A-1(L) is a Myoviridae cyanophage isolated in 1970s9 that specifically infects the model cyanobacterium Anabaena sp. PCC 7120. Using cryo-electron microscopy (cryo-EM), we solved the structure of A-1(L) tail machine, which consists of three parts: a 205-Å-long neck, a 1045-Å-long contractile tail with a complicated baseplate, and six pairs of tail fibers. The dodecameric gp2 portal, the pentadecameric gp5 and the hexameric gp7 sequentially constitute the neck of A-1(L), to which five neck fibers are attached. The long and contractile tail of A-1(L) contains 24 rings of gp10 hexamers that form the tube, surrounded by the sheath of 24 helically stacked gp9 hexamers.

The central spike/trimeric gp25, hub/trimeric gp15, six monomeric gp16, and six wedges/heterotrimeric (gp31)2-gp32 form a compact baseplate at the distal end of the tail. The central spike locates at the innermost of baseplate, each subunit of which adopts a conserved structure: an N-terminal α-helix, an oligonucleotide/oligosaccharide binding fold, a consecutive β-strand domain and a C-terminal loop. The N-terminal α-helices (residues Met1-Arg30) of three gp25 subunits form a tripod to interwind with the tripod of three C-terminal helices (residues Pro666-Ala689) of TMP via hydrogen bonds and hydrophobic interactions. The two interwound tripods are surrounded by the trimeric hub, each subunit of which adopts an architecture different from the previously reported hub proteins. Besides the conserved barrel domain that is commonly found in most myophages, the hub of A-1(L) possesses three extra domains. Using in vitro enzymatic activity assays with the commercially available lysozyme as the positive control, we found that the endoglucanase and peptidase domains of hub/gp15 can hydrolyze Anabaena sp. PCC 7120 cells. Six gp16 subunits adopt two conformations (termed gp16A and gp16B), which alternatively anchor on the hub to connect the internal trimeric hub and external hexameric wedge. The C-terminal tail (residues Ile126-Asp152) of gp16A deeply inserts into the barrel domains of hub, whereas that of gp16B forms a four-stranded antiparallel β-sheet with the α/β domain of tube initiator. Moreover, the N-terminal tail (residues Met1-Leu20) of gp16 runs downwards to recruit the heterotrimeric wedge, which is composed of two gp31 subunits with different conformations (termed gp31A and gp31B) and one gp32 subunit at the periphery. The insertion domain (residues Glu81-Gly180) of gp31A inserts in a cleft on the hub, whereas that of gp31B stretches outside to hold the LTF.

>[3x]MQDPIIKILIGNDTFLLGQEIIDLDFQIGEGKKQNNINFTIFDKDGFFADKYISTSYAQGGIDLPIDFLENPDDAKDTNSASTATEVDSVGNGTVSRSGVFTPKIRAFLDTIASKETAPGTALNIEGYRSVSGSSTLFDESEMVAGGFPRSQGSKNIGRYQFTVIDYNHARSKYPNINNYSPQNQDLLAYFKLQHRNVLPYLLRDDLDNAIDKASYEWASFPGIGKPQGQFNQVQSGTTIASLKSYYETRLAYYRSLEAGSDFQASAPKDTTNNQYAGKEYKTIRTLSNSTTASFYGYNDGFDSSDLTANGERFNPEGITAAHESLPFGTLVKVTWAVNNKSVVVRINDRGAFVRLGRQIDLSYGAAKALSSPGNDAIAAGLLTVKLEVVELRTPIGENLKESAKNQIAENLEKIKKNQKELATPEISAKGTQITLEVSIDRSAIAVFSFLHTGTKHNAIISDTTTFTGQSVNWVLNRRVKNTRYTGVTLKGLAATITRQYGLDLDMSEEGEMIENISQVSQTDWQFLEKMTAIQGFGMRTVGKVLQIYKITVNAKKLNYTISVVDNVKSLIVTDQAQTDATGSSQKIEHYGGRMTTVVDADSGSLIKVDKDNKREAGSAARTFTTGVDVPQPQIQKQYSNPRPEGASVKEFQLQLELHTSQSDLENLTPDTALYIENTLPFIVGKSWFIESVRHSFSEGIFTSQVSAYIPVAPKAIATDSGEQNSVVFDNSQSASQGVGKLPVYEILSYRSGRTVKKITSLQQSYEHWRGTGGYTAYKQLSGFSSPVSYMKGRPNQLVYDFILQQNGNQSCPVPSPASGRVVATGGSNGMVKIDTGGGEVRLLHMSNIRVKPGQNVIRGTILGTQASVGGTSTGTHLHIEANQFILESYVQSLVTGNW;>MIVDEFSSVYECLLYCYKMVKRSEQLNGRRVFPILSVVTNNNDPEGRRRVKIADPLFGNLIESNWIRPIRVSQNQDNPLPQINQMVIVWFVDGDSEKGYYLPIINDANPSREKDDPVNDSAVRIEGNNTIRIDKNDSETVGGNQTVAIAGEQNINVDGNLIENIGGDIDQNVTGKIEVRSESTILIDADGTIIIKNDSGAFISLGGNGEVLIQDSQGRKIRLGGAFNSTWDLNGLPMAFINATSVTIAGKQIATVGAVDTRGDTIVNKGW[3x];>[3x]MANRQHVISVDLRLLTGNFDSSLNYIQGRLNGVFGVVSDNATNSFFGNGGFLSSYLWNQAFNAIQMAGIAAFRAIGNEVKRAISYQDNLISMATSYKGLLNLTTKEAFGLARESNIIFQQRNVGLPTFGNFGTQLRAQYGDDFLSAFYDQNNMKGSLERTADMIGRTTVLLGSISGVTNYQRTSFLSNFLSDDFKKLQRLEVFRNSPQLQRAFNSQVDSIGGEQGFNALTRKDRLLLLENIAAIAVDDDIIKAYKDSLGGVLSRLGQELFGDIGIFSFTRDLIFGLPNTSILNSITFFMKEVFAPDGVFGLIKPALQGIVDTVLIGTKFILDRTSFIFMGLNALARVLQPIAPLIYATSSALTVLAAVGLANTIKSAVQGYLISSGAAMLGGRMGMAAMFGMGGDLVGLKTLGTLGLGKLIAPLGFLTMGLDKLADVGWLAISGGFAKAALGIKTFGMSLWAIVANPAFLTIAGIVGAIALAGYTLWKYWEPIGDFLQGFWIGFKAGLPILDQIESVLQSIGQALSPITEGFKNMASAMQPVLDGFTKFFNLQQEKGGENYVKQGVNFGDAASGVTRTILSNPLINPFSGFFGLFGNPAQNKADGDPQSVMSAINDERRKMPSGASLVIANSSENVFTRSQTQQLASAGRGSTVINNTFNISGADPQAIAKQIADIINSQWQGTLTDYA;>MTTQEFLSKNKTIESELLDLLIKPNTDDSILTRNKQAIADRDLFDIEWEPGQSLNKLATEYLGDSFAWQIIADANGIDPTKEIDIGAGLKVPDQKALENSIKKFIVNSPTGKQLISDAKQSILNLIGVGDSNTEFSKTLKDCIGKVVNFSFDNTQ[6x];>MSKFLKNRAVVNGLPVIKNPGKYQHCYLIEYEDSTNVKQTPTENKNKQQQGFPVYLFMMNPENITYNLPINYQEIAIPFTAKNQLNYSNGGNIVMTMSNLILDTMDEKRSLQPLIDRLIALREPTVKKGLKSHPKILAFKWGSNTFAPCVLTNISFDVTRWIDGYPTKARVNMSLKEIQKPSSDSKALEEAKKKVKVETVQNGNLKKTLSEKQLIDGVKRVTEYLKKNISFQPRTIQNILSDPKSVIKIDKDTGQVSLFNGNGEFAALVGTYNGDIFSPSRQ[6x];>[6x]MYVYPPRIINGTLYKSTDLAEYTRGKILQTLSIVRGELVADPFFGVPLRLFSNINDYQSDVSKIQIILEEEITEAQFIVTGDLKNNGIVSLTVYWAYLGTENIENFEIDTSNIF;>[12x]MTTDLNAPQLVVDDYEQLIIDSLVHTNVVSNGEFTDLDASGFMRPFAGTMAYAGSELLYKANLASIAAAKSFFKNVLGVPEDTGTKATTTLQFGLSASLSTDFIVPINFQVSDLSGTLRFYTIGNLVIPAGATFGTIEAIAEDIGEKYNVSANFIDQYSTPLTYLQYVTNIRPATNGRSGETIDNLIERCAQIIRIRNPVSALDFEQLAELTMGEGSRCKAIGLLGINKIVTDPQPGVVHLFLLDVNGNPADPVTISTVGATLQPRIMLGTRLLISPMEVLNIELELIALSDSSKTFQQLADDILEALKVFFNPANLTPGEPVLIEEVKFAIRSVGGLSISYLQMNDNAINIPMPNQWTIPRFSYIGFELTDSEGTVYRDNVVTVTNPEE;>[6x]MSKDAFTAWNVDRRPIYSRMPKEQVGTSYHDYIATDWLTAYWDKIFIECYDKLEDLPRQFDPLQCDEEYLDFLAPLCGWTAPYWSGDYPPESKRVLLANSYSLIWRDKGSLTVLSFVLNALFINHRIFVPGSFILGQSQVSEDTLGAAGWEFEILLPRDYAENGYEFRLTLKIASLFSPLWCKYRVRYDNL Profilin is an ubiquitous cytoskeletal protein that interacts with several molecules, such as actin, proline-rich ligands, and phosphoinositides to perform several cellular functions. Profilin is also an important allergen present in pollen grains, food plants, and rubber tree, and it is considered a pan-allergen, because it is present in all eukaryotic cells and is therefore involved in allergic cross-reactions. In this work, we focus on the study of two plant pan-allergens, profilins from the rubber tree (rHev b 8) and maize (rZea m 12), in their monomeric and dimeric forms. Here we isolated the monomeric and dimeric species of the recombinant profilin allergens rHev b 8 and rZea m 12 and obtained their crystallographic 3D structures.

The rHev b 8 and rZea m 12 crystals (5 mg/mL) were obtained using the conditions described in the materials and methods section. These crystals diffracted to resolutions of 1.9 and 2.2 Å, respectively, and belonged to the P43212 space group. A backbone alignment of the two 3D-structures reveals that they adopt the same conformation, with a root-mean-square-deviation (rmsd) of 0.27 Å. The sequence alignment shows that the principal differences are between residues 37ANFPQFKSEEITGIMSDFH55for rHev b 8 and 37ENFPELKPEEVAGMIKDFD55 for rZea m 12. These residues are structurally located in a region exposed to the solvent, mainly in the loop that connects β-strand 2 and α-helix 2, but some also belong to α-helix 2. The assays showed that mAb 2F5 specifically recognizes monomeric rHev b 8, even at a low concentration (2 μg/mL); conversely, mAb 2F5 showed no reactivity towards monomeric rZea m 12, suggesting that this IgE recognizes a conformational epitope on the surface of rHev b 8 that is not shared with rZea m 12. Interestingly, the flexible loop and α-helix 2 do not participate in the establishment of the rHev b 8 dimer interface and the competitive ELISAs between monomeric and dimeric rHev b 8 confirmed that this region is exposed for interaction with mAb 2F5. However, between the monomeric and dimeric forms of both allergens we observed a significant difference in the IgE binding (P < 0.001), which suggests that the monomer has additional IgE epitopes in the region that establishes the homodimer interface. When the cells were stimulated with monomeric rHev b 8 using the same and two fold the concentration of the dimer (130 and 260 nM, respectively) the release of β-hexosaminidase reached near half of the homodimer, and the positive controls responses P < 0.001.

> MSWQAYVDDHLMCEIEGNHLSAAAIIGQDGSVWAQSANFPQFKSEEITGIMSDFHEPGTLAPTGLYIGGTKYMVIQGEPGAVIRGKKGPGGVTVKKTNQALIIGIYDEPMTPGQCNMIVERLGDYLIDQGY> MSGGSPAEREAGRIVVRGDVAIAEAVVRKVGEVAGKEVILLISYRKNGEWITYQRNLEATPEDVERTIAVIREIYEESGGDFILAIFSDPEVGAAGRAVAAAAAGGSGSHHWGSTHHHHHH;> I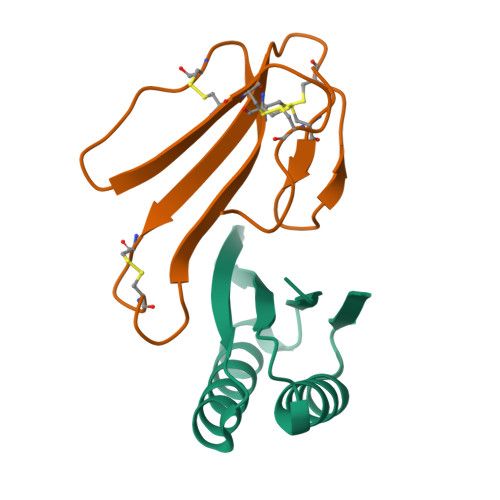RCFITPDITSKDCPNGHVCYTKTWCDAFCSIRGKRVDLGCAATCPTVKTGVDIQCCSTDNCNPFPTRKRP> TENILRKSDEEIQKEITARVKALESMLIEQGILTTSMIDRMAEIYENEVGPHLGAKVVVKAWTDPEFKKRLLADGTEACKELGIGGLQGEDMMWVENTDEVHHVVVCTLCSCYPWPVLGLPPNWFKEPQYRSRVVREPRQLLKEEFGFEVPPSKEIKVWDSSSEMRFVVLPQRPAGTDGWSEEELATLVTRESMIGVEPAKAVHHHHHH;> MNGVYDVGGTDGLGPINRPADEPVFRAEWEKVAFAMFPATFRAGFMGLDEFRFGIEQMNPAEYLESPYYWHWIRTYIHHGVRTGKIDLEELERRTQYYRENPDAPLPEHEQKPELIEFVNQAVYGGLPASREVDRPPKFKEGDVVRFSTASPKGHARRARYVRGKTGTVVKHHG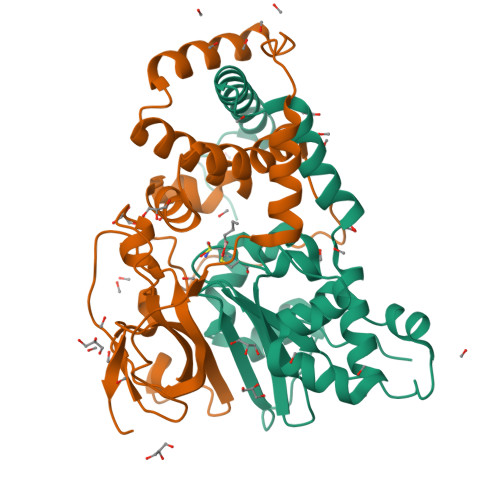AYIYPDTAGNGLGECPEHLYTVRFTAQELWGPEGDPNSSVYYDCWEPYIELVDTKAAAA> MVQQLSLFGSIGDDGYDLLISTLTTISGNPPLLYNSLCTVWKPNPSYDVENVNSRNQLVEPNRIKLS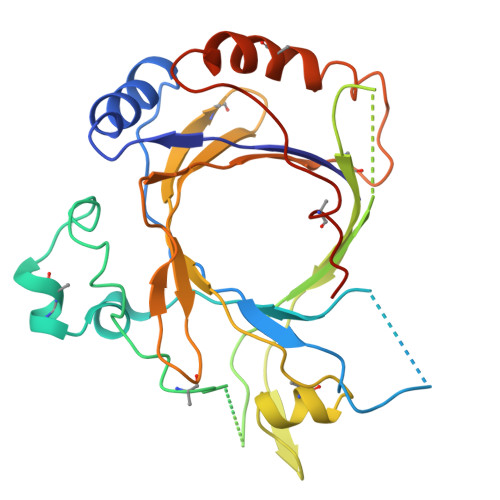KEVPFSYLIDETMMDKPLNFRILKSFTNDKIPLNYAMTRNINSDDIIDVDMDASPAPSNESCSPWSLQISDIPAAGNNRSVSMQTIAETIILSSAGKNSSVSSLMNGLGYVFEFQYLTIGVKFFMKHGLILELQKIWQIEEAGNSQITSGGFLLKAYINVSRGTDIDRINYTETALMNLKKELQGYIELSVPDRQSMDSRVAHGNILI>[4x]MKILKTLTLRGPNYWSIRRKKLIVMRLDLEDLAERPSNSIPGFYEGLIKVLPSLVEHFCSPGYQGGFLERVKEGTYMGHIVQHVALELQELVGMTAGFGRTRETSTPGVYNVVYEYVDEQAGRYAGRAAVRLCRSLVDTGDYPRLELEKDLEDLRDLGANSALGPSTETIVTEAEARKIPWMLLSARAMVQLGYGVYQQRIQATLSSHSGILGVELACDKEGTKTILQDAGIPVPRGTTIQYFDDLEEAIND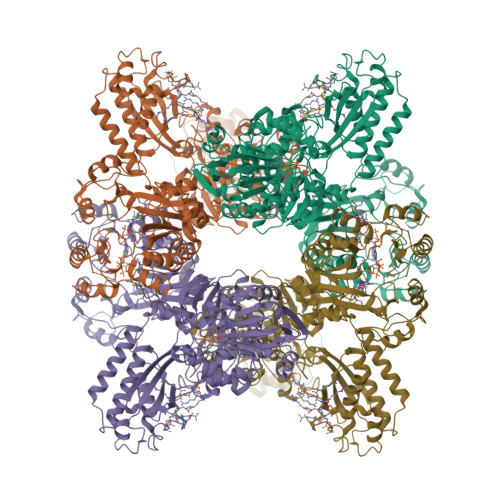VGGYPVVIKPLDGNHGRGITINVRHWQEAIAAYDLAAEESKSRAIIVERYYEGSDHRVLVVNGKLVAVAERIPAHVTGDGSSTISELIEKTNQDPNRGDGHDNILTKIVVNKTAIDVMERQGYNLDSVLPKDEVVYLRATANLSTGGIAIDRTDDIHPENIWLMERVAKVIGLDIAGIDVVTSDISKPLRETNGVIVEVNAAPGFRMHVAPSQGLPRNVAAPVLDMLFPPGTPSRIPILAVTGTNGKTTTTRLLAHIYRQTGKTVGYTSTDAIYINEYCVEKGDNTGPQSAGVILRDPTVEVAVLETARGGILRAGLAFDSCDVGVVLNVAADHLGLGDIDTIEQMAKVKSVIAEVVDPSGYAVLNADDPLVAAMADKVKAKVAYFSMNPDNPIIQAHVRRNGIAAVYESGYLSILEGSWTLRVEQAKLIPMTMGGMAPFMIANALAACLAAFVNGLDVEVIRQGVRTFTTSAEQTPGRMNLFNLGQHHALVDYAHNPAGYRAVGDFVKNWQGQRFGVVGGPGDRRDSDLIELGQIAAQVFDRIIVKEDDDKRGRSEGETADLIVKGILQENPGASYEVILDETIALNKALDQVEEKGLVVVFPESVTRAIDLIKVRNPIGENLYFQ;>DDDDDDDDDDDDDDDD[8x]>EVSTTQNDTLKVMTHNVYMLSTNLYPNWGQTERADLIGAADYIKNQDVVILNEVFDNSASDRLLGNLKKEYPNQTAVLGRSSGSEWDKTLGNYSSSTPEDGGVAIVSKWPIAEKIQYVFAKGCGPDNLSNKGFVYTKIKKNDRFVHVIGTHLQAEDSMCGKTSPASVRTNQLKEIQDFIKNKNIPNNEYVLIGGDMNVNKINAENNNDSEYASMFKTLNA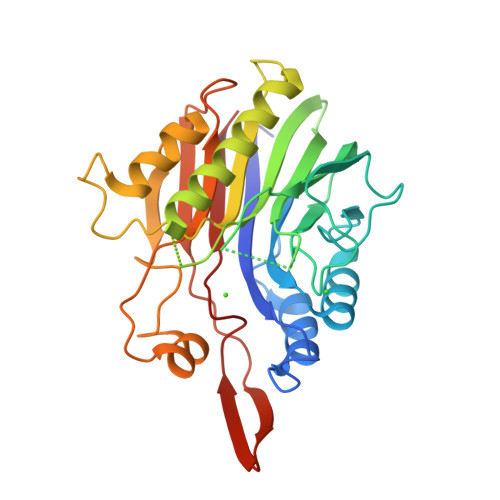SVPSYTGHTATWDATTNSIAKYNFPDSPAEYLDYIIASKDHANPSYIENKVLQPKSPQWTVTSWFQKYTYNDYSDHYPVEATISMK[4x]>[4x]GPLGSKIVRIEKARDIPLGATVRNEMDSVIISRIVKG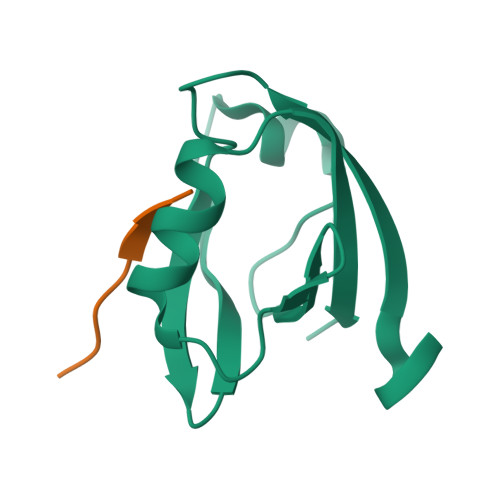GAAEKSGLLHEGDEVLEINGIEIRGKDVNEVFDLLSDMHGTLTFVLIPSQ;>[4x]SRVPDLLV>[2x]MTIENMSVNKSFGGWHKQYSHQSQTLNCEMRFAIYLPPQASSGKKVPVLYWLSGLTCTDENFMQKAGAQALAAELGIAIVAPDTSPRGENVADDEGYDLGKGAGFYVNATQAPWNRHYRMYDYVVDELPKLIESMFPVSDKRSIAGHSMGGHGALVIALRN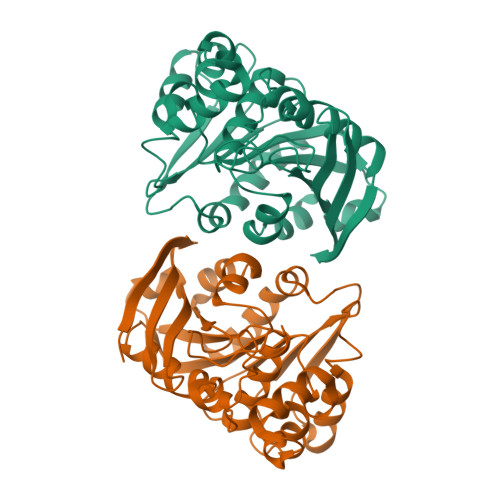ADAYQSVSAFSPISNPINCPWGKKALTAYLGRDSATWMEYDASVLMRQATQFVPALVDQGDADNFLVEQLKPEVLEAAAKVKGYPLELNYREGYDHSYYFISSFIENHLRFHAEHLGK eCGP123 is a bright green FP engineered for extreme stability, and was developed using a two-step process. Phanta was isolated by expression screening of a library targeting amino acid positions 62/63/65/69 and 191/192/193 in the bright green fluorescent protein eCGP123. Phanta contains the substitutions Gln62Met, Thr69Val and His193Gln. The protomers in each protein are typical of the GFP-superfamily and consist of an 11-stranded β-barrel (or β-can) with two small helices forming interconnecting loops protecting the chromophore from bulk solvent.

In contrast, eCGP123T69V underwent very efficient reversible photoswitching (~ 92% photoswitching depth) and had ~ 10 fold increased OFF rate. The chromophores in eCGP123H193Q and eCGP123T69V are essentially coplanar with the 4-hydroxybenzyl ring twisted out of plane relative to the imidazolinone ring by only 4.6° and 1.8°, respectively averaged across all four protomers. In eCGP123T69V the imidazole ring of His193 stacks against the 4-hydroxybenzyl ring forming a π-π interaction. Presumably the histidine is charged as it interacts with side chains of the conserved Glu148 and Glu215. In eCGP123T69V and eCGP123 the side chains of His193, Glu215, Glu148, Arg66 and a water (H2O91) form a planar network of hydrogen bonds and salt bridges beneath the chromophore. Although the Thr69Val substitution results in reorientation of the Arg66 side chain in eCGP123T69V, the water (H2O91) changes position maintaining the network of interactions beneath the chromophore observed in eCGP123. The aliphatic side-chain of the valine substitution in eCGP123T69V can no longer hydrogen-bond with the Nε of Arg66 allowing the NNH1/NH2 of Arg66 to extend towards the imidazolinone O2 forming a direct hydrogen bond and a water (H2O144) mediated hydrogen-bond. Closer interaction of the Arg66 side chains with the imidazolinone ring would increase charge stabilisation on the ring. By comparison, eCGP123 contained a single species decaying with a fluorescence lifetime of 2.3 ns whilst eCGP123T69V contained a major and minor species with a fluorescence lifetime of 1.33 ns and 2.62 ns, respectively. It is possible that the chromophore environment of eCGP123T69V can exist in two emissive conformations although the structural data appears to show evidence of single conformation.

>[4x]MSVIKPEMKIKLRMEGAVNGHKFVIEGEGIGKPYEGTQTLDLTVKEGAPLPFSYDILTPAFQYGNRAFVKYPKDIPDYFKQAFPEGYSWERSMTYEDQGICIATSDITMEGDCFFYKIRFDGTNFPPNGPVMQKKTLKWEPSTEKMYVRDGVLKGDVNMALLLEGGGHYRCDFKTTYKAKKDVRLPDAHEVDHRIEILSHDKDYNKVRLYEHAEARYSMLPSQAKASGKPIPNPLLGLDSTHHHHHH>[2x]GPGHMVVKFSYMWTINNFSFCREEMGEVIKSSTFSSGANDKLKWCLRVNPKGLDEESKDYLSLYLLLVSCPKSEVRAKFKFSILNAKGEETKAMEDQRAYRFVQGKDWGFKK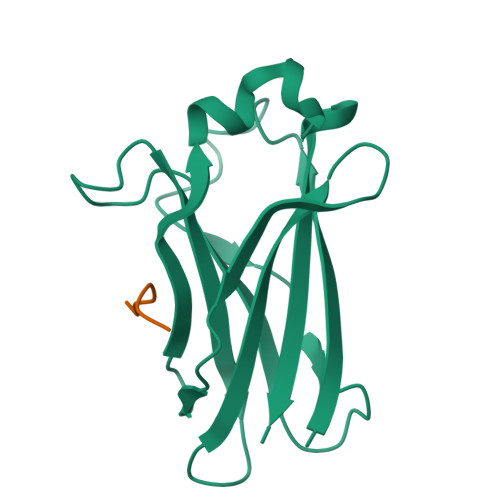FIRRDFLLDEANGLLPDDKLTLFCEVSVVQD;>PATPTASSSSSTTPT[2x]> SNAIAVGSERSADGKGMLLANPHFPWNGAMRFYQMHLTIPGRLDVMGASLPGLPVVNIGFSRHLAWTHTVDTSSHFTLYRLALDPKDPRRYLVDGRSLPLEEKSVAIEVRGADGKLSRVEHKVYQSIYGPLVVWPGKLDWNRSEAYALRDANLENTRVLQQWYSINQASDVADLRRRVEALQGIPWVNTLAADEQGNALYMNQSVVPYLKPELIPACAIPQLVAEGLPALQGQDSRCAWSRDPAAAQAGITPAAQLPVLLRRDFVQNSNDSAWLTNPASPLQGFSPLVSQEKPIGPRARYALSRLQGKQPLEAKTLEEMVTANHVFSADQVLPDLLRLCRDNQGEKSLARACAALAQWDRGANLDSGSGFVYFQRFMQRFAELDGAWKEPFDAQRPLDTPQGIALDRPQVATQVRQALADAAAEVEKSGIPDGARW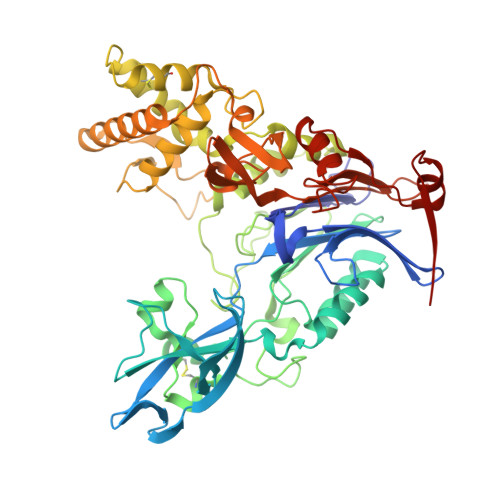GDLQVSTRGQERIAIPGGDGHFGVYNAIQSVRKGDHLEVVGGTSYIQLVTFPEEGPKARGLLAFSQSSDPRSPHYRDQTELFSRQQWQTLPFSDRQIDADPQLQRLSIRE> GIDPFTKYKVERNPPAFTELQLPRYIMAGFPVCPKLSLEFGDPASSLFRWYKEAKPGAAEPEVGVPSSLSPSSPSSSWTETDVEE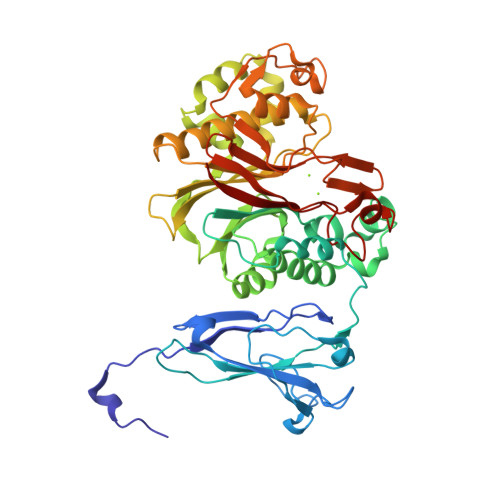RVYTPSNADIGLRLKLHCTPGDGQRFGHSRELESVCVVEAGPGTCTFDHRHLYTKKVTEDALIRTVSYNILADTYAQTEFSRTVLYPYCAPYALELDYRQNLIQKELTGYNADVICLQEVDRAVFSDSLVPALEAFGLEGVFRIKQHEGLATFYRKSKFSLLSQHDISFYEALESDPLHKELLEKLVLYPSAQEKVLQRSSVLQVSVLQSTKDSSKRICVANTHLYWHPKGGYIRLIQMAVALAHIRHVSCDLYPGIPVIFCGDFNSTPSTGMYHFVINGSIPEDHEDWASNGEEERCNMSLTHFFKLKSACGEPAYTNYVGGFHGCLDYIFIDLNALEVEQVIPLPSHEEVTTHQALPSVSHPSDHIALVCDLKWK Archaeal DNA polymerases from the B-family (polB) have found essential applications in biotechnology. Variants of the archaeal polymerase from Thermococcus gorgonarius, TgoT, that can either generate HNA from DNA (TgoT_6G12) or DNA from HNA (TgoT_RT521) have been previously identified. In this study, six X-ray structures of DNA and HNA polymerases are reported: (i) three apo- structures of TgoT, TgoT_6G12, and TgoT_RT521-; (ii) two DNA-bound structures of TgoT_6G12 in binary and ternary complexes; and (iii) one DNA-bound structure of TgoT_6G12, which has incorporated two HNA nucleotides. Consistent with all other DNAPs from B-family, TgoT and its variants fold into five distinct structural subdomains.

TgoT_6G12 polymerase corresponds to TgoT variant with 14 supplementary mutations (V589A, E609K, I610M, K659Q, E664Q, Q665P, R668K, D669Q, K671H, K674R, T676R, A681S, L704P, and E730G). To better understand how the mutations added on TgoT variants impact the structure of the polymerase, the X-ray structures of the apo form of TgoT, replicative polymerase TgoT_6G12, and reverse transcriptase TgoT_RT521 were solved by crystallography. Crystals were obtained for the three polymerases and diffracted at 2.4, 3.1, and 2.35 Å, respectively. Comparison of TgoT_6G12 with TgoT_RT521 structures shows a strong similarity between the two polymerases (r.m.s. deviation for Cα atoms: 0.6 Å). The final apo TgoT_6G12 and TgoT_RT521 structures contained flexible segments in the thumb subdomains. The high flexibility of these segments probably results from the absence of DNA or HNA inside the active site. On the contrary, larger rigid-body movements in the palm domains (r.m.s. deviation for Cα atoms: 2.7 Å for TgoT_RT521 and 2.3 Å for TgoT_6G12) were observed. However, very large rigid-body movements can be locally seen between the thumb subdomain of TgoT and those of TgoT_6G12 and TgoT_RT521. For example, between amino acids 619 to 660, for TgoT_RT521, the r.m.s. deviation for Cα is 9.4 Å and between amino acids 619 and 650 for TgoT_6G12, it is 7.9 Å.

> MILDTDYITEDGKPVIRIFKKENGEFKIDYDRNFEPYIYALLKDDSAIEDVKKITAERHGTTVRVVRAEKVKKKFLGRPIEVWKLYFTHPQDQPAIRDKIKEHPAVVDIYEYDIPFAKRYLIDKGLIPMEGDEELKMLAFAIATLYHEGEEFAEGPILMISYADEEGARVITWKNIDLPYVDVVSTEKEMIKRFLKVVKEKDPDVLITYNGDNFDFAYLKKRSEKLGVKFILGREGSEPKIQRMGDRFAVEVKGRIHFDLYPVIRRTINLPTYTLEAVYEAIFGQPKEKVYAEEIAQAWETGEGLERVARYSMEDAKVTYELGKEFFPMEAQLSRLVGQSLWDVSRSSTGNLVEWFLLRKAYERNELAPNKPDERELARRRESYAGGYVKEPERGLWENIVYLDFRSLYPSIIITHNVSPDTLNREGCEEYDVAPQVGHKFCKDFPGFIPSLLGDLLEERQKVKKKMKATIDPIEKKLLDYRQRLIKILANSFYGYYGYAKARWYCKECAESVTAWGRQYIETTIREIEEKFGFKVLYADTDGFFATIPGADAETVKKKAKEFLDYINAKLPGLLELEYEGFYKRGFFATKKKYAVIDEEDKITTRGLKMVRRDWSEIAKETQARVLEAILKHGDVEEAVRIVKEVTEKLSKYEVPPEQLVIYQPITKQLHDYRARGPHVSVAKRLAARGIKIRPGTVISYIVPKGSGRIGDRAIPFDEFDPAKHKYDAGYYIENQVLPAVERILRAFGYRKEDLRYQKTRQVGLGAWLKPKT WW domains organize molecular assemblies by binding to short, proline rich peptide motifs each with ~4–6 residues. The type I WW domains bind to a consensus ‘PPxY’ motif (where P is proline, x is any amino acid and Y is tyrosine, also known as PY-motif) with very modest affinities (with Kd in the range of a few to a few tens of µM). To achieve this goal, we determined the high resolustion structures of 7 representative WW tandem/target complexes, and measured the binding constants of >100 WW domain tandems or isolated WW domains binding to known or previously unknown targets. In this study, we discovered that WW tandems, but not individual WW domains, can bind to target proteins with extremely high affinity and with very high sequence specificity.

We were able to obtain high diffraction quality crystals when the Dendrin PY23 sequence was fused to either the N- or C-termini of the YAP WW tandem. We solved the structures of these two versions of the complex. Although each WW domain engages the ‘PPxY’ motif following the canonical type I WW/target bindings, the overall structure of the YAP WW tandem/Dendrin PY23 complex differs substantially from those of the KIBRA/MAGI2 WW tandems in complex with the same ligand (Figure 3E vs Figure 3F for example) in two distinct aspects. First, the inter-domain linker of the YAP WW tandem is unstructured and there is no C-terminal helix following YAP WW2. Thus, the two WW domains of YAP do not form a supramodule due to very limited inter-domain contact. This is supported by the two versions of the complex structures solved, in which the inter-domain orientations are obviously different. Second, the Dendrin PY23 binds to the YAP WW tandem in a parallel orientation (i.e. PY2 binds to WW1 and PY3 binds to WW2), instead of the antiparallel binding orientation observed for the KIBRA/MAGI2 WW tandems. This is again likely attributed by the lack of inter-domain interactions between the two WW domains of YAP so that each domain can freely choose its more preferred PY-motif. In contrast, the coupling between WW1 and WW2 in YAP is minimal. Therefore, the target binding synergism between the two WW domains in the YAP tandem is also low. For example, the binding of YAP WW tandem to Dendrin PY23 is only a few tens tighter than the isolated WW domains (Figure 4D2 and Supplementary file 1B and D), and this relatively low synergism likely originates from the very closely spaced PY-motifs of Dendrin PY23.

>[2x]GPGSDRPPPYVAPPSYEGPHRTLGVPLPAGWEMAKTSSGQRYFLNHNDQTTTWQDPRKAMLSQLNVPAPASPAVPQTLMNSASGPLPDGWEQAMTQDGEVYYINHKNKTTSWLDPR PHOSPHORIC ACID MONO-(3-HYDROXY-PROPYL) ESTER | C3 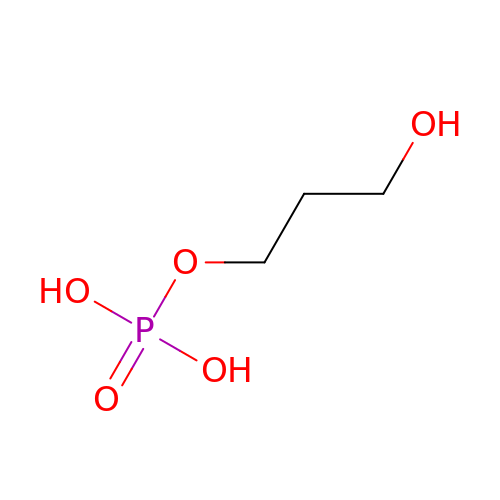H9 O5 P | HYCSHFLKPSMPGO-UHFFFAOYSA-N Capping protein (CP), also known as CapZ in muscle cells and Cap32/34 in Dictyostelium discoideum, plays a major role in regulating actin filament dynamics. CP is a ubiquitously expressed heterodimer comprising an α- and β-subunit. It tightly binds to the fast growing end of actin filaments, thereby functioning as a “cap” by blocking the addition and loss of actin subunits. Vertebrates contain two somatic variants of CP, one being primarily found at the cell periphery of non-muscle tissues while the other is mainly localized at the Z-discs of skeletal muscles.

We here report the first high resolution structure of a cytoplasmic CP. The overall structure of Cap32/34 from Dictyostelium discoideum reveals a similar arrangement as compared to its sarcomeric variant CapZ. Superposition of the two Cap32/34 molecules within the asymmetric unit revealed only small deviations in their overall structures, with a root-mean-square deviation (r.m.s.d.) of 0.3 Å for 512 common Cα atoms. Briefly, Cap32/34 has the shape of a mushroom, comprising a stalk (“N-stalk”) and a cap (“central β-sheet” and “antiparallel H5s”). The mushroom stalk is composed of six anti-parallel α-helices, of which three are contributed from the N-terminus of each subunit (H1–3). The cap consists of a single ten-stranded antiparallel β-sheet formed by five β-strands of each subunit (S6–10). In Cap34 the region located opposite to the C-terminal β-tentacle moves towards the antiparallel helices that interconnect the heterodimer leading to a more compact CP structure. In contrast to the α-tentacle, neither Cap32/34 nor CapZ crystals grown at physiological pH provided an interpretable electron density for the C-terminal segment of the β-subunit (β-tentacle), indicating that this part of the CP molecule is highly mobile. The sequence alignment further reveals that Lys-142 and Lys-143 of Cap32 are C-terminally flanked by three additional residues (Gly-144, Gln-145, Pro-146) resulting in an elongated linker region. Since “linker βS7–S8” provides a positively charged surface close to the basic patch on CP, it might participate in the initial electrostatic binding to acidic regions on the barbed end of actin filaments.

>[2x]MASNQELVQIATNFLLNAPPCEFMEVVSDVRALLPSESLLNASAGSTFREYNTSQMVSVQTSKGSALITKEGEISNNEYLDPKNKQVITYDHIKQEVTGERSASGEIEQDIEQYRAAFDEEATKYCNEYYPNGVSAVYGTKVSEGIKITVCISTCIYKPNAFYSGRWRSVWTCTFKPGSGNVTSNGKVQVNVHYFEDGNVQLNTVTQKQTTSPSADAQSTAVNAFKAIGKAELNLHTALDNNYSTMGDTTFKALRRALPINRTKINWQKVKNFKIANELNK;>MDHHHHHHHHTSETGYVQGTEKQLSCCLDLMRRLPPSQIEDNLAGLLDLVPDLTEDLLSSIDQPLKVAYDAVSKKDYLLCDYNRDADSYRSPWSNKYDPPLSGACYPSSKLRDIEVQANEIFEIYLNLYFEGGVSSVYCWDLDDNFAAVVLMKKTQDQSKKGQPMRGTWDSIHVVEVKLGKKDKAVYKLTSTVMLSIETDNDNTGKVNLAGSLTRQDEKEYTFNEVDTHCVNIGKMVEDMESKLRQTLETIYFGKTKEVVNTLRNATGNSELEKRKNLSNQIGSAIGNRG[2x]> MSQQENPKYLWWNHRIIPWEEATVHLTDYWWASVTAVFEVISGYWNNAEGEMYIFRLEDHARRLEQSMQLIRMPKEFTVDEICQATIDLVRANDYRGDVFIMPLAYAVGNKAFRVVGDRTTEMFIYSRPAVSRLEEDFSLHACYSSWTRINERVLPPRIKALANYRNSQLASSEAAMNGYDTALFLNPEGKVAEGTGSCVFFVRKGKLITPDITSGILESITRDTVIHLAREVLGLEVEERVVDRTETYLADEAFLCGTHAEITPIASIDRHEMKHGAPGPITRQLRDIYRE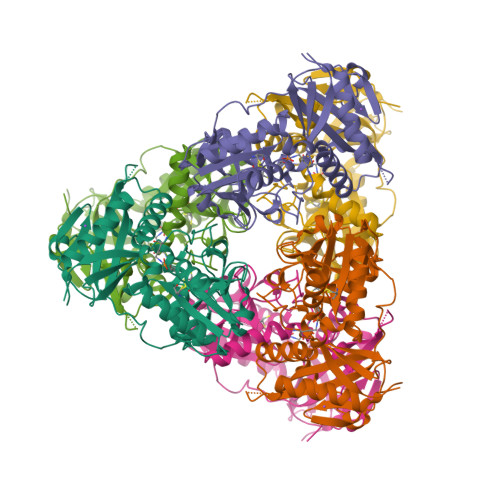VVYGRDFRYRNWLTPVGMGVRAEQ>MDLTNKNVIFVAALGGIGLDTSRELVKRNLKNFVILDRVENPTALAELKAINPKVNITFHTYDVTVPVAESKKLLKKIFDQLKTVDILINGAGILDDHQIERTIAINFTGLVNTTTAILDFWDKRKGGPGGIIANICSVTGFNAIHQVPVYSASKAAVVSFTNSLAKLAPITGVTAYSINPGITRTPLVHTFNSWLDV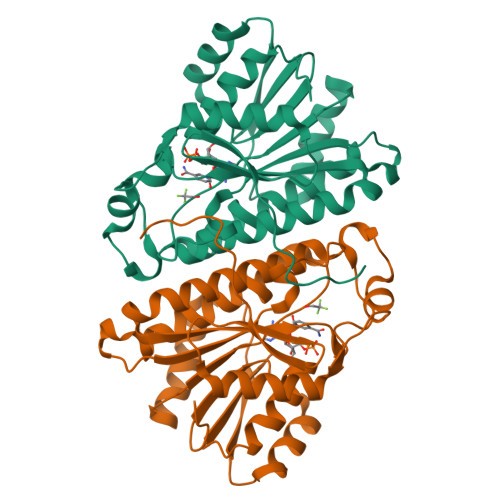EPRVAELLLSHPTQTSEQCGQNFVKAIEANKNGAIWKLDLGTLEAIEWTKHWDSHI[2x]2-O-phosphono-alpha-D-glucopyranose 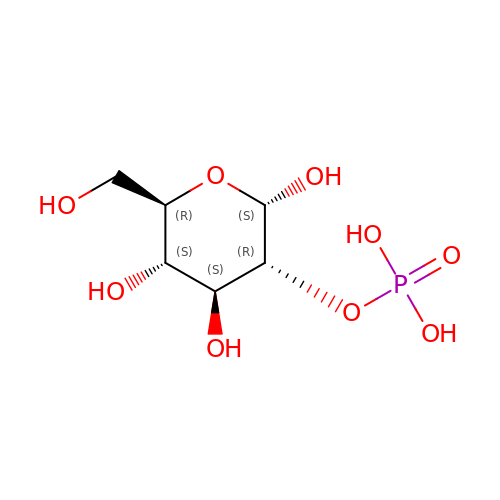| C6 H13 O9 P | SIUIENVKPUKAHD-DVKNGEFBSA-N[(2-{[(2S)-1-{(2S,4S)-4-[(7-{2-[(3R)-2,6-dioxopiperidin-3-yl]-1-oxo-2,3-dihydro-1H-isoindol-4-yl}hept-6-yn-1-yl)oxy]-2-[(2R)-2-phenylmorpholine-4-carbonyl]pyrrolidin-1-yl}-3,3-dimethyl-1-oxobutan-2-yl]carbamoyl}-1-benzothiophen-5-yl)di(fluoro)methyl]phosphonic 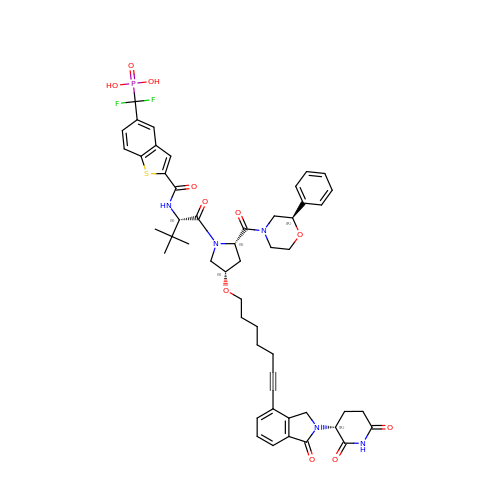acid | C51 H56 F2 N5 O11 P S | BOMRVPKXCINUMI-ZEGZQYLTSA-N>MSAPKPFVIGIAGGTASGKTTLAQALARTLGERVALLPMDHYYKDLGHLPLEERLRVNYDHPDAFDLALYLEHAQALLRGLPVEMPVYDFRAYTRSPRRTPVRPAPVVILEGILVLYPKELRDLMDLKVFVDADAD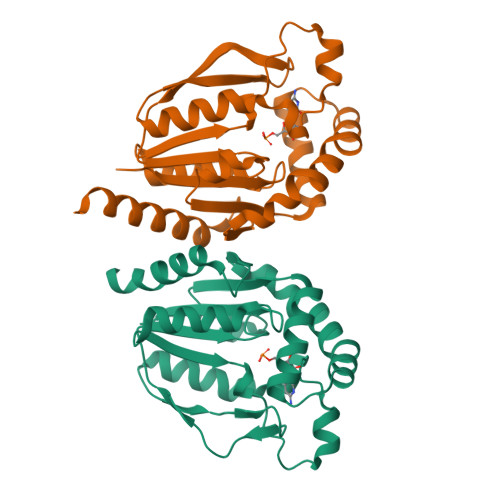ERFIRRLKRDVLERGRSLEGVVAQYLEQVKPMHLHFVEPTKRYADVIVPRGGQNPVALEMLAAKALARLARMGAA[2x]> MAAAAVSSAKRSLRGELKQRLRAMSAEERLRQSRVLSQKVIAHSEYQKSKRISIFLSMQDEIETEEIIKDIFQRGK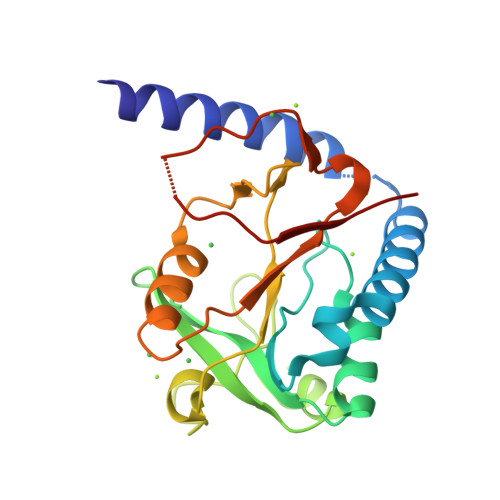ICFIPRYRFQSNHMDMVRIESPEEISLLPKTSWNIPQPGEGDVREEALSTGGLDLIFMPGLGFDKHGNRLGRGKGYYDAYLKRCLQHQEVKPYTLALAFKEQICLQVPVNENDMKVDEVLYEDSSTA Seb1 has two ordered domains, a CID at the N-terminus and an RRM-containing RNA-binding region closer to the C-terminus. In contrast to this widely accepted paradigm, we demonstrate that the fission yeast CID-RRM protein Seb1 drives transcription termination of both types of Pol II transcribed genes. Using a multidisciplinary approach, our study demonstrates that conserved CID-RRM proteins play a key role in 3′ end formation of Pol II transcripts. We present high-resolution structures of the CID and RRM domain of Seb1.

Thus, we crystallized the Seb1-CID1–152 and compared the structure with other CID structures in complex with CTD peptides to determine whether interacting aa are topologically conserved. The highest affinity was observed to S2P, followed by S5P, S7P and unphosphorylated peptide. Also, several aa make phosphate-independent contacts with the CTD. Most notably, a Tyr (Y64 in Seb1) forms an aromatic (π–π) interaction with Y1 of the CTD in all published CTD-CID structures (Y62 in Fig. 2e and Y67 in Fig. 2f) and a conserved Asp was shown to be important for Nrd1 function. When these two residues are mutated to Ala, binding to S2P-CTD can still be observed (lanes 7 and 9) suggesting that both aa may contribute to the S2P interaction. Y64 and D67 were predicted to be involved in phosphorylation-independent interactions and to therefore affect binding to all types of CTD. Indeed, Y64K reduces binding to all phosphorylated and unphosphorylated peptides; however, it has a stronger effect on S2P than S5P interaction (lane 4 and Fig. 2g–i). Despite Seb1 having its highest affinity to S2P-CTD, this demonstrates that disrupting interactions with S2P-CTD alone is not sufficient to observe the full phenotype, and that interactions with S5P-CTD are also required for proper functioning of Seb1.

> MSGIAEFDGILDSLEHSKTGISGSKILKLTNLSMENVSENAQFVASVYKYAKRAPVTHKLGALYILDSIVRSFQDGAKKNNESFENPVDASFSGGWCKAAEITDSLVADAIQHAPSAHLPKILKLCDIWEKASTFPPEKLESLRSKLKDAMALEHHHHHHHH>[4x]DSISLSLINEGPSYASKVSVGSNKQQQTVIIDTGSSDFWVVDSNAQCGKGVDCKSSGTFTPSSSSSYKNLGAAFTIRYGDGSTS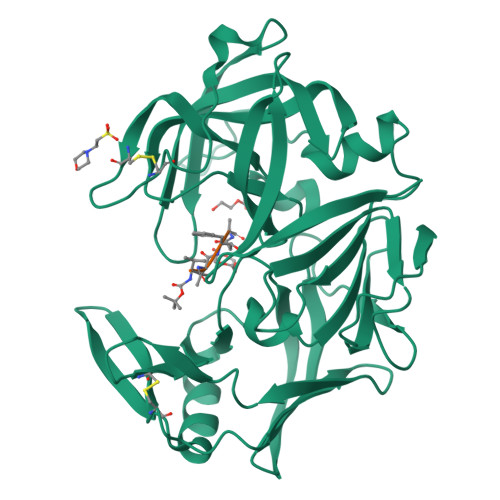QGTWGKDTVTINGVSITGQQIADVTQTSVDQGILGIGYTSNEAVYDTSGRQTTPNYDNVPVTLKKQGKIRTNAYSLYLNSPSAETGTIIFGGVDNAKYSGKLVAEQVTSSQALTISLASVNLKGSSFSFGDGALLDSGTTLTYFPSDFAAQLADKAGARLVQVARDQYLYFIDCNTDTSGTTVFNFGNGAKITVPNTEYVYQNGDGTCLWGIQPSDDTILGDNFLRHAYLLYNLDANTISIAQVKYTTDSSISAV;>[4x]VVFAFA>[2x]GPASPDRFAVSAEAENKVREQQPHVERIFSVGVSVLPKDCPDNPHIWLQLEGPKENASRAKEYLKGLCSPELQDEIHYPPKLHCIFLGAQGFFLDCLAWSTSAHLVPRAPGSLMISGLTEAFVMAQSRVEELAERLSWDFTPGPSSGASQCTGVLRDFSALLQSPGDAHREALLQLPLAVQEELLSLVQEASSG

Zinc finger antiviral protein (ZAP) binds CpG dinucleotides in viral RNA and targets them for decay. ZAP interacts with several cofactors to form the ZAP antiviral system, including KHNYN, a multidomain endoribonuclease required for ZAP-mediated RNA decay. KHNYN contains three structural domains, an N-terminal KH domain, a PilT N-terminal (PIN) nuclease domain, and a C-terminal CUElike domain (also known as a CUBAN domain) that binds ubiquitin and NEDD8 (18, 21, 22, 23). Here, we demonstrate that the KHNYN amino-terminal extended-diKH (ex-diKH) domain is required for antiviral activity and present its crystal structure.

The asymmetric unit contains two copies of the ex-diKH domain. In each copy, the domain spans residues 12 to 198 and is composed of an N-terminal type 1 KH module (KH1, residues 12–74), a short linker (residues 75 and 76), a second type 1 KH module (KH2, residues 77–144), a longer linker (residues 145–161) and a C-terminal bundle (CTB) extension composed of three alpha helices (residues 162–198). The KH2 domain has the expected β1-α1-α2-β2-β3-α3 type 1 KH topology but in KH1 α1 and α2 are near continuous constituting α1′ that contains a pronounced proline kink surrounding P29. Inspection of the domain packing within the protein revealed a substantial interdomain interface that packs KH1 onto KH2. At the center of the interface, these include hydrophobic packing of KH1 side chains I34, F35, Y69, and L73 with A104, H110, L124, and A127 of KH2. These are accompanied by surrounding salt bridges and hydrogen bonding between R33 and D101, R65 and the mainchain carbonyl of S106 and between Y69 and H110, with R33 also π-stacking with W105. Additionally, the CTB extension packs onto the KH2 domain making an interface stabilized by multiple interactions between CTB α8 and KH2 α5, including a salt bridge network between E196 and R134, R134 and E189 and R141, as well as hydrogen bonding between R141 and the carbonyl of the mainchain A185. The computed Complex Formation Significance Score of 0.0 also suggested that the interface is unlikely to have biological relevance. This conclusion is supported by solution size-exclusion chromatography coupled to multiangle laser light scattering (SEC-MALLS) data that revealed that the ex-diKH domain was exclusively monomeric over the range of concentrations tested (0.5–8 mg/ml). Therefore, the dimer observed in the crystal likely is a result of crystal packing rather than any residual assembly associated with an ex-diKH domain homo-oligomerization function. Further analysis of the interresidue contacts in the ex-diKH crystal structure identified exposed arginine residues, R33 and R65, that make salt bridges and cation–π stacking interactions at the edge of the KH1-KH2 cleft that potentially could form part of a protein binding site.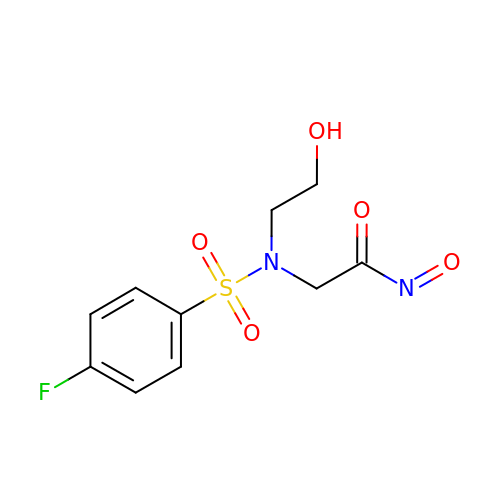2-[(4-fluorophenyl)sulfonyl-(2-hydroxyethyl)amino]-N-oxo-ethanamide | C10 H11 F N2 O5 S | XNNFYDODDRKLAF-UHFFFAOYSA-N Galectins (Gals) are a family of animal lectins that bind β-galactose-containing glycoconjugates, and their carbohydrate recognition domain (CRD) has a conservative amino acid sequence. To date, 16 mammalian galectins have been discovered, and galectin-7 (Gal-7; also termed p53-induced gene 1 product), belonging to prototype galectins, is a multifunctional effector by productive pairing with distinct glycoconjugates and protein counter-receptors in the cytoplasm and nucleus, as well as on the cell surface. Gal-7 participates in diverse processes, such as controlling apoptosis, cell migration and cell adhesion. Gal-7 was crystallized in complex with glycerol under two different conditions.

The two refined structures, structure 1 (homodimeric Gal-7 binds two glycerol molecules) and structure 2 (homodimeric Gal-7 binds three glycerol molecules), were crystallized using two different conditions, one at a relatively low concentration of PEG3350 (12%) and the other at a higher concentration (20%). Homodimeric Gal-7 binds three glycerol molecules at its two carbohydrate recognition binding sites (GOL A and GOL B) and the new binding pocket formed by its N-terminal and loop connecting strands S2 and F1 (GOL C), respectively. Monomer A of structure 2 can bind two glycerols. Its N-terminal (Asn 3-Val 4) and loop connecting strands S2 and F1(Val 124-Leu 130) form a GOL C-binding pocket. GOL C can form hydrogen bonds with Val 4 and Gly 126, respectively. In addition, GOL C interacts indirectly with Val 128 and Leu 130 through a water molecule in the new ligand binding pocket of Gal-7. This means that the N-terminal of Gal-7 interacts with loop connecting strands S2 and F1 via a hydrogen bond bridge formed between GOL C and a molecule of water. Discrepancies between structure 1 and structure 2 in monomer A are due to the absence or presence of GOL C. B-factors of structure 1 suggests that the N-terminal regions are very flexible, while the N-terminal region of structure 2 is relatively stable due to the binding of GOL C. Glycerol binds the pocket near the N-terminus of Gal-7, which can greatly reduce the flexibility and improve the stability of this region. It is noted that glycerol binds to GOL C sites of monomer A but not monomer B in structure 2. In addition, we found the GOL C pocket, which binds glycerol in structure 2 of Gal-7, is deep and negatively charged with surrounding amino acids.

>MSNVPHKSSLPEGIRPGTVLRIRGLVPPNASRFHVNLLCGEEQGSDAALHFNPRLDTSEVVFNSKEQGSWGREERGPGVPFQRGQPFEVLIIASDDGFKAVVGDAQYHHFRHRLPLARVRLVEVGGDVQLDSVRIF[2x]> GSPGISGGGGGSHIEGYECQPIFLNVLEAIEPGVVCAGHDNNQPDSFAALLSSLNELGERQLVHVVKWAKALPGFRNLHVDDQMAVIQYSWMGLMVFAMGWRSFTNVNSRMLYFAPDLVFNEYRMHKSRMYSQCVRMRHLSQEFGWLQITPQEFLCMKALLLFSIIPVDGLKNQKFFDELRMNYIKELDRIIACKRKNPTSCSRRFYQLT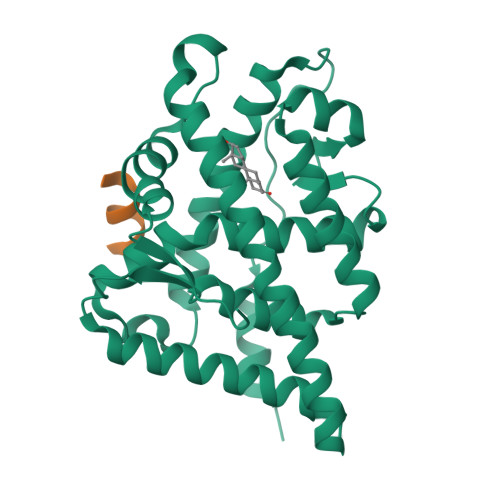KLLDSVQPIARELHQFTFDLLIKSHMVSVDFPEMMAEIISVQVPKILSGKVKPIYFHTQ;> SSRGLLWDLLTKDSRSGSGK>MISTKVTINCPAGLDSKAAALLVQKVSKYSSSIWLEKGERRANAKSLLGLLSLGVERNAAITIITDGEDEKKAADEISEYFTVGFH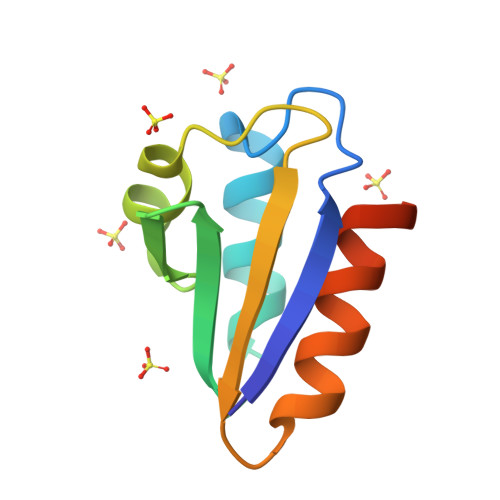HHHHH[3x]3'-chloro-4'-(alpha-D-mannopyranosyloxy)biphenyl-4-carbonitrile | C19 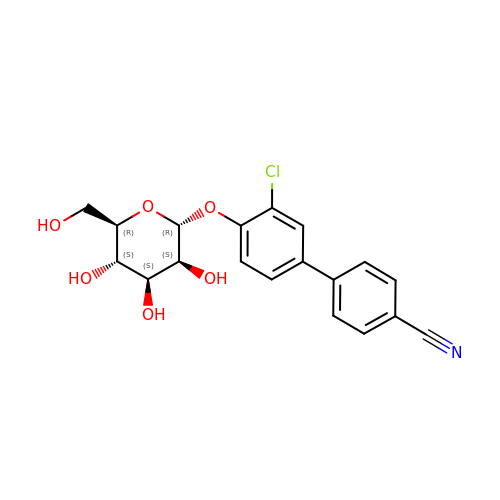H18 Cl N O6 | NJQGFQIHQPLUNX-GFEQUFNTSA-N> MGGSRSRKSDQGIIAGNVPLTPIQKWFFGKNFTNTGHWNQSSVLYRPEGFDPKVIQSVMDKIIEHHDALRMVYQHENGNVVQHNRGLGGQLYDFFSYNLTAQPDVQQAIEAETQRLHSSMNLQEGPLVKVALFQTLHGDHLFLAIHHLVVDGISWRILFEDLATGYAQA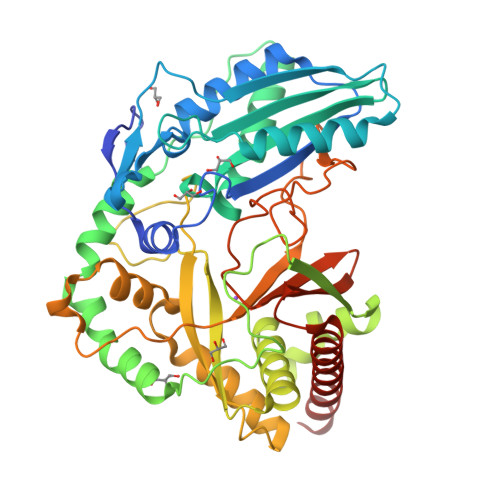LAGQAISLPEKTDSFQSWSQWLQEYANEADLLSEIPYWESLESQAKNVSLPKDYEVTDCKQKSVRNMRIRLHPEETEQLLKHANQAYQTEINDLLLAALGLAFAEWSKLAQIVIHLEGHGREDIIEQANVARTVGWFTSQYPVLLDLKQTAPLSDYIKLTKENMRKIPRKGIGYDILKHVTLPENRGSLSFRVQPEVTFNYLGQFDADMRTELFTRSPYSGGNTLGADGKNNLSPESEVYTALNITGLIEGGELVLTFSYSSEQYREESIQQLSQSYQKHLLAIIAHCLQSHHHHHH> XXXXXXXXXXXSLKHLYSSIILIKNSRDESSSPYEWCIWQLKRCFAHQIETPQEVIPIIISVSSMDNKLSSRIIQTFCNLKYLKLDELTLKKVCGGILPLWKPELISGTREFFVKFMASIFMWSTRDGHDNNCTFSETCFYVLQMITNWVLDDKLIALGLTLLHDMQSLLTLDKIFNNATSNRFSTMAFISSLDILTQLSKQTKSDYAIQYLIVGPDIMNKVFSSDDPLLLSAACRYLVATKNKLMQYPSTNKFVRMQNQYIMDLTNYLYRNKVLSSKSLFGVSPDFFKQILENLYIPTADFKNAK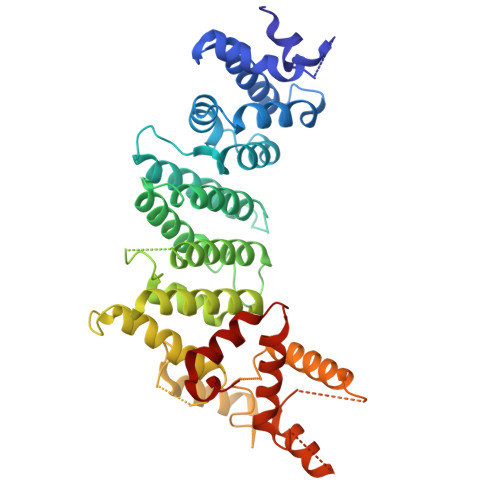FFTITGIPALSYICIIILRRLETAENTXXXXXXXXXXXXXXXXXXXXXXXXXXXXXXXXXXXVNNIHDLRVKILMHLSNTANPYRDIAAFLFTYLKSLSKYSVQNS> MKKLLPILIGLSLSGFSSLS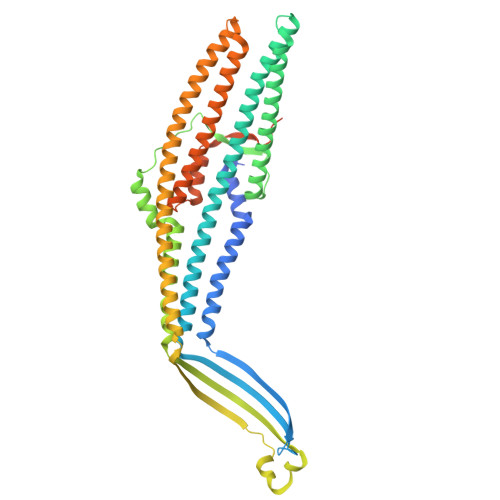QAENLMQVYQQARLSNPELRKSAADRDAAFEKINEARSPLLPQLGLGADYTYSNGYRDANGINSNATSASLQLTQSIFDMSKWRALTLQEKAAGIQDVTYQTDQQTLILNTATAYFNVLNAIDVLSYTQAQKEAIYRQLDQTTQRFNVGLVAITDVQNARAQYDTVLANEVTARNNLDNAVEQLRQITGNYYPELAALNVENFKTDKPQPVNALLKEAEKRNLSLLQARLSQDLAREQIRQAQDGHLPTLDLTASTGISDTSYSGSKTRGAAGTQYDDSNMGQNKVGLSFSLPIYQGGMVNSQVKQAQYNFVGASEQLESAHRSVVQTVRSSFNNINASISSINAYKQAVVSAQSSLDAMEAGYSVGTRTIVDVLDATTTLYNAKQELANARYNYLINQLNIKSALGTLNEQDLLALNNALSKPVSTNPENVAPQTPEQNAIADGYAPDSPAPVVQQTSARTTTSNGHNPFRN The functional core proteins of the signal recognition particle (SRP) and the SRP receptor (SR) (called Ffh and FtsY in bacteria) contain GTPase domains and form a distinct subfamily of GTPases. These GTPases mediate cotranslational targeting of secretory and membrane proteins to the endoplasmic reticulum (ER) membrane in eukaryotes or the plasma membrane in prokaryotes. SRP GTPases are unique in that activation of GTP-hydrolysis occurs upon formation of a complex of two GTPases. Here we report the structures of two conformations of FtsY in complex with the substrate analogue GMPPNP.

In addition, apo crystals of FtsY pre-derivatized with chloromercurial nitrophenol (CMNP) were grown and solved by multiple wavelength anomalous diffraction (MAD) and used as a molecular replacement model for the apo/GMPPNP dimer forms. Finally, in the ground state apo FtsY, the position of the guanine specifying Asp258 is further extended than in F1 or F2. Interestingly, the interaction distance between Lys256 and Asp229 is maintained but the interaction with the the P-loop is decreased by more than 1 Å. In apo FtsY, the IBD has re-structured and as a consequence Arg142 and Gln148 have returned to the active site although their positions differ from the active form. By superimposing bound nucleotide from the active form, F1 and F2, a clash in the van der Waals spacing between the apo position of this motif II arginine sidechain and the γ phosphate position of bound nucleotide is observed (not shown). In addition, Gln148 has rotated clockwise (from the same reference axis as above) greater than 2 Å from the active position to locate itself again out of the active site but in the opposite relative direction than in F1 and F2. In apo FtsY Arg195 is positioned away from the phosphate-binding cavity. The preceding glycine, Gly194, forms a salt bridge with the P-loop and orients the backbone nitrogens away from the γ phosphate.

>[2x]MGFFDRLKAGLAKTRERLLKAIPWGGNLEEVLEELEMALLAADVGLSATEEILQEVRASGRKDLKEAVKEKLVGMLEPDERRATLRKLGFNPQKPKPVEPKGRVVLVVGVNGVGKTTTIAKLGRYYQNLGKKVMFCAGDTFRAAGGTQLSEWGKRLSIPVIQGPEGTDPAALAYDAVQAMKARGYDLLFVDTAGRLHTKHNLMEELKKVKRAIAKADPEEPKEVWLVLDAVTGQNGLEQAKKFHEAVGLTGVIVTKLDGTAKGGVLIPIVRTLKVPIKFVGVGEGPDDLQPFDPEAFVEALLED>[2x]MSDESNP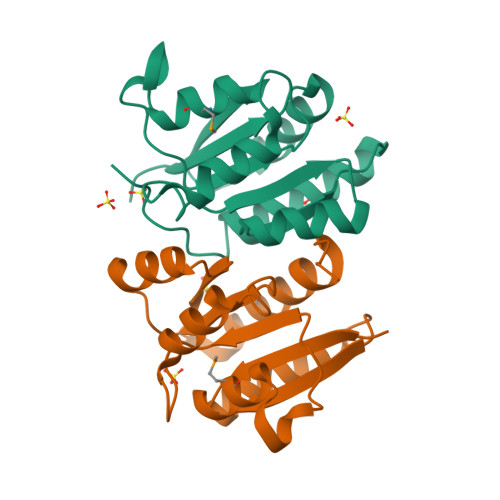PKVILLVEDSKADSRLVQEVLKTSTIDHELIILRDGLAAMAFLQQQGEYENSPRPNLILLDLNLPKKDGREVLAEIKQNPDLKRIPVVVLTTSHNEDDVIASYELHVNCYLTKSRNLKDLFKMVQGIESFWLETVTLPAAPG>[2x]SMLDRELESSAPGVPSVSVHPLLGSHVVLPQEPEEHLWQGDVGTEAHPWLSDHRVHQVAVLPGAAYCEMALA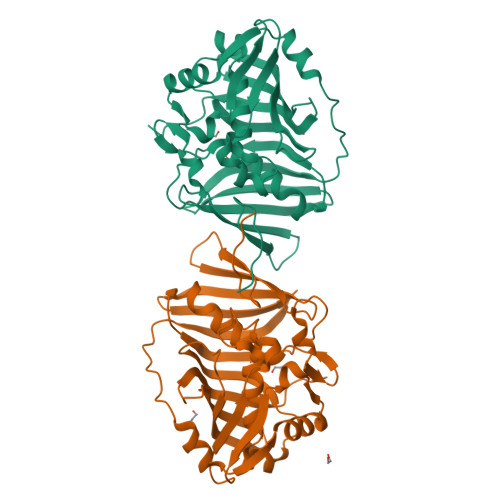AVTPVLGDTGEVHDLKFHDMLLLDDATPVWVSAAVTAPGTAEFGVETHQSGDRTQRATAVLRGDVDAERPAAHSIDALLAAHPNRVDGDELRAGFGTVGIGHGAAFAGLSEAYVATAAEPTVVAAVALPGPLRSGQRGYTVHPALLDACFQSVIAHPEVQNIASGMLLPLGVRRLRAYGSTRNVRYCLSRIVKADSFGVEADLELLDADGTVLLSAMGLQLGTGNSDKAEEER>MGPSGNDGLEGVSYIPYKDIVGVWTVCHGHTGKDIMLGKTYTKAECKALLNKDLATVARQIN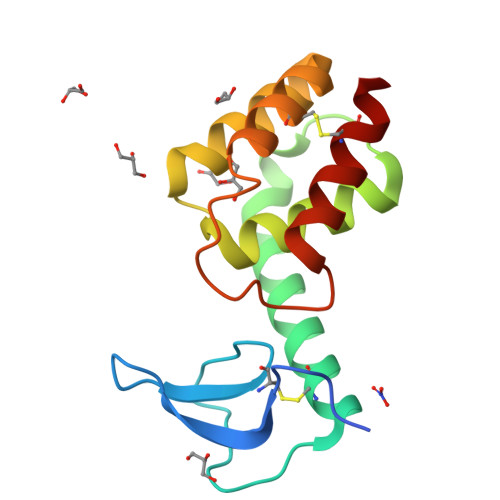PYIKVDIPETMRGALYSFVYNVGAGNFRTSTLLRKINQGDIKGACDQLRRWTYAGGKQWKGLMTRREIEREICLWGQQ[2x]> 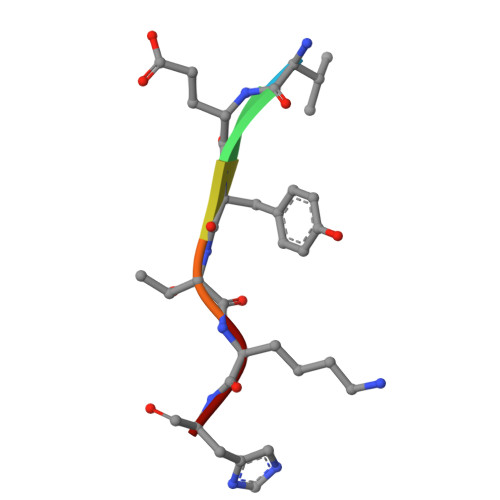VEYTKH> LPQILNDEEISLYSFYDYANKNFNIEKLKQKDDIFSYQESEIESSLLVHSDAEQTEVAVEIFSKVLHYMNSNPLVSK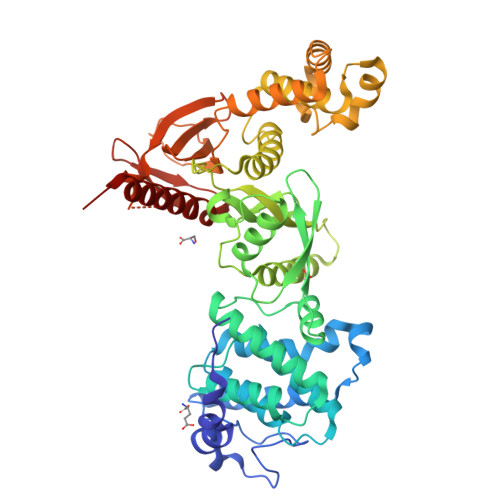KDPADFYSPVKFILTKGLAIESLRDEIYCQLIKQSTSNPIQDLNIRVWELIHFTCSTFPPTRKLIKYFAAYLKTTIQQSDVSKSVKDSAQASYFILQRFTLNGARKQVPSVTELESIKENRPIFVRITATDGSLKGLHIDSATTCQESSNDLSQRSRMRVNSKENGFTIIESFNGIERDIAPTDKLCDVLSKVENLQATLSSKIQVNFKFVFKKKLFFDNITNNVPTTSINVENEFYYHQLFNDLFNSNYCKDQDYQISIGSLKLQFESSDYTDEIRAWLPGNGRGKYFTTDIEKNRFDDFINKYKSHKGLSPEDAKKQMVQLLEKHPLANCSLVVCEHQSESLPYPKNFVLALNVNGINIYDPATSKMLESVKYSNQSQQNLKSDDKSSVSIILENKSTLQAFTGDVQKLVSLIKEYSLYLRNNALEHHHHHH> AQSVPYGVSQIKAPALHSQGYTGSNVKVAVINSGIDSSHPDLNVAGGASFVPSETNPFQDNNSHGTHVAGTVLAVAPSASLYAVKVLGADGSGQYSWIINGIEWAIANNMDVINMSLGGPSGSAALKAAVDKAVASG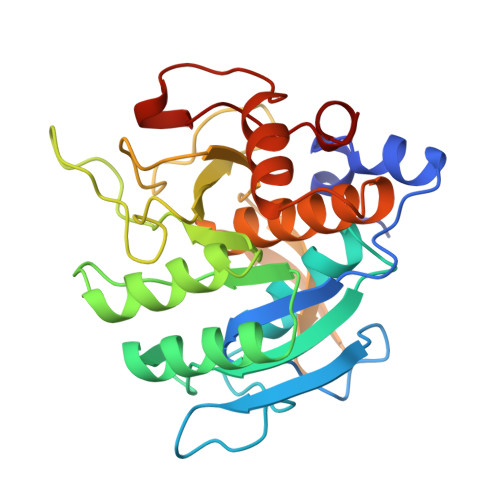VVVVAAAGNEGTSGSSSTVGYPGKYPSVIAVGAVDSSNQRASFSSVGPELDVMAPGVSIVSTLPGNKYGAKSGTAMASPHVAGAAALILSKHPNWTNTQVRSSLENTTTKLGDSFYYGKGLINVQAAAQ>[2x]GAMVSQPIKLLVGLANPGPEYAKTRHNAGAWVVEELARIHNVTLKNEPKFFGLTGRLLIN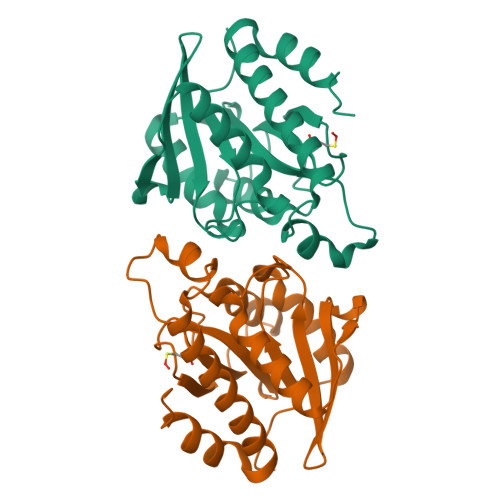SQELRVLIPTTFMNLSGKAIAALANFYQIKPEEIMVAHNELDLPPGVAKFKQGGGHGGHNGLKDTISKLGNNKEFYRLRLGIGHPGHKDKVAGYVLGKAPAKEQECLDAAVDESVRCLEILMKDGLTKAQNRLHTFKAE>[2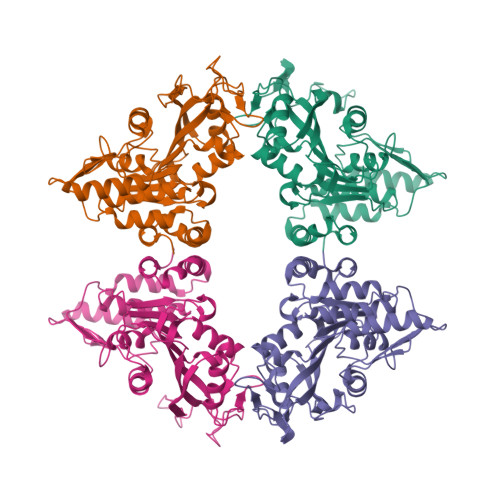x]MMFNFANFYQLIAQDTRLQPWLNVLPQQLTDWQNAEHGDFPRWLKALNKIPEGAPDQIDIKHSVTISNDTPFHQGELKKLESLLRTFHPWRKGPYTVHGIHIDTEWRSDWKWDRVLPHISPLKNRSVLDVGCGNGYHMWRMLGEGARLCVGIDPSHLFLIQFEAIRKLMGGDQRAHLLPLGIEQLPKLEAFDTVFSMGVLYHRRSPLDHLIQLKDQLVSGGELILETLVIEGDETAVLVPKERYAQMRNVYFFPSARALKVWLELVGFEDVRIVDENVTSVDEQRTTNWMTHNSLPDYLDQNDPSKTVEGYPAPRRAILVAKKPGHHHHHHG> VYTLPAGADFIMCYS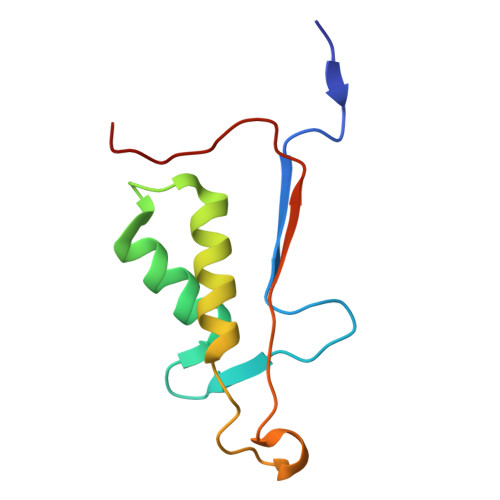TAEGYYSYRETVNGSWYIQDLCEMLKKYGSELEFTEILTLVNRKVSLRSVPNCKDPAAIGKKQMPCFASMLTKKLYFRPK>GPLGSKASNNDDHNYVYPLPENMVYRFNKSTNILDYLSTERDHVMMAVQYYMSKQRLDDLYRQLPTKTRSYIDIINMYCDKVNNDYNRDMNIMYDMASTESFTVYDINNEVNTILMDNKGLGVRLATISFITELGKRCMNPVETIKMFTLLSHTICDDCFIDYITDIS[6x];>PSSTMGQVGRQ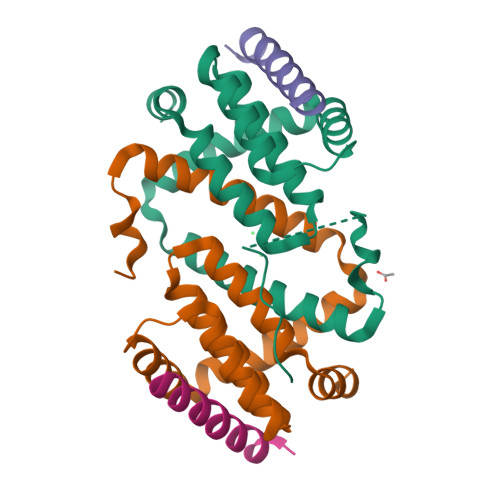LAIIGDDINRRYDSE[6x]>[4x]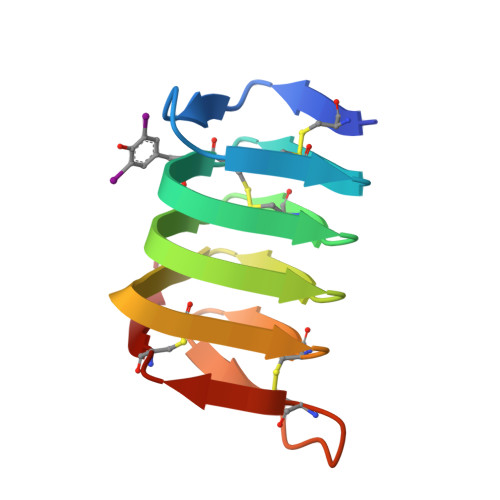DGSCTNTNSQLSANSKCEKSTLTNCYVDKSEVFGTTCTGSRFDGVTITTSTSTGSRISGPGCKISTCIITGGVPAPSAACKISGCTFSAN> GFDSWHPPAPGDRRG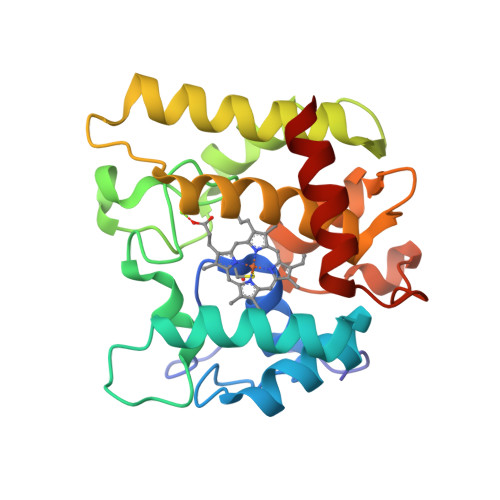PCPMLNTLANHGFLPHNGRNITKEITVNALNSALNVNKTLGELLFNFAVTTNPQPNATFFDLDHLSRHNILEHDASLSRADYYFGHDDHTFNQTVFDQTKSYWKTPIIDVQQAANARLARVLTSNATNPTFVLSQIGEAFSFGETAAYILALGDRVSGTVPRQWVEYLFENERLPLELGWRRAKEVISNSDLDQLTNRVINA> MDCRNLCGAAAPSRLVQPGCFICRGVAVSIPPAAPGPATSVFDTPPSTFSLRPDGTIIAGTGIRGDHASVGTDGTIEMFIVPFIGDVTGSELTHPYA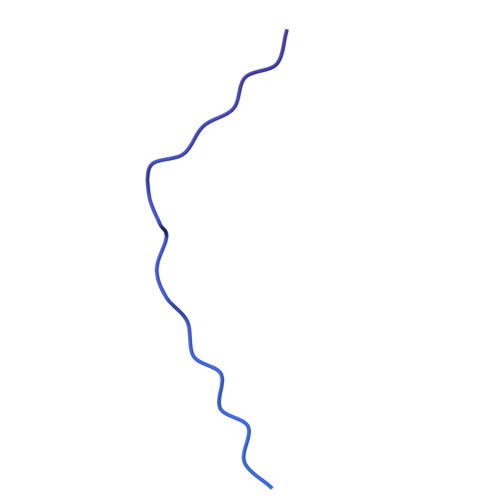VELQDGEELAIAFGVTLKSGYGARITEYYDVSLFLENGGNSKELTLQPANTKSGYVWSDGHGYNITDSDGDLHTVQNVTRPVWFEMTEPGIVGVIMEARYKATGLVSSSISITVNVTYAD> MEQNPQSQLKLLVTRGKEQGYLTYAEVNDHLPEDIVDSDQIEDIIQMINDMGIQVMEEAPDADDLMLAENTADEDAAEAAAQVLSSVESEIGRTTDPVRMYMREMGTVELLTREGEIDIAKRIEDGINQVQCSVAEYPEAITYLLEQYNRVEAEEARLSDLITGFVDPNAEEDLAPTATHVGSELSQEDLDDDEDEDEEDGDDDSADDDNSIDPELAREKFAELRAQYVVTRDTIKAKGRSHATAQEEILKLSEVFKQFRLVPKQFDYLVNSMRVMMDRVRTQERLIMKLCVEQCKMPKKNFITLFTGNETSDTWFNAAIAMNKPWSEKLHDVSEEVHRALQKLQQIEEETGLTIEQVKDINRRMSIGEAKARRAKKEMVEANLRLVISIAKKYTNRGLQFLDLIQEGNIGLMKAVDKFEYRRGYKFSTYATWWIRQAITRSIADQARTIRIPVHMIETINKLNRISRQMLQEMGREPTPEELAERMLMPEDKIRKVLKIAKEPISMETPIGDDEDSHLGDFIEDTTLELPLDSATTESLRAA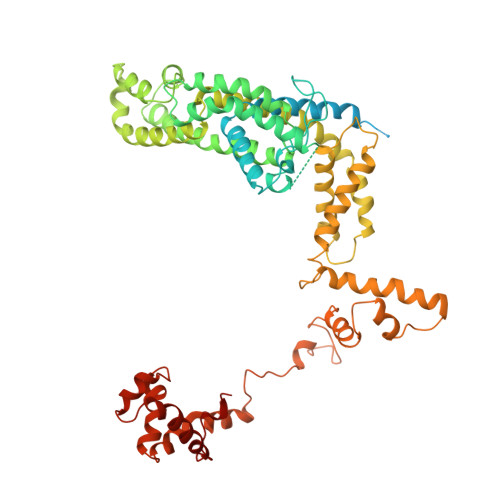THDVLAGLTAREAKVLRMRFGIDMNTDHTLEEVGKQFDVTRERIRQIEAKALRKLRHPSRSEVLRSFLDD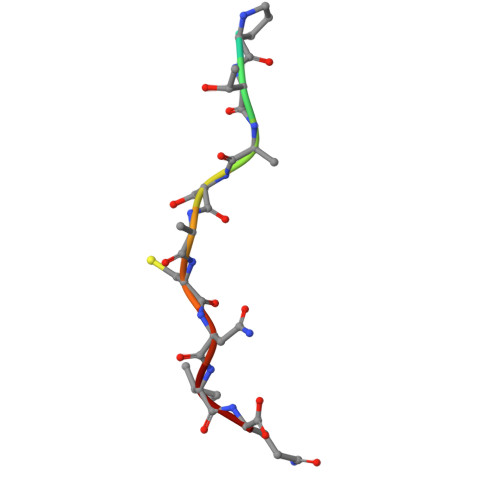> DDPTASACNIQ>HHHHHHENLYFQGDTKEQRILNHVLQHAEPGNAQSVLEAIDTYCEQKEWAMNVGDKKGKIVDAVIQEHQPSVLLELGAYCGYSAVRMARLLSPGARLITIEINPDCAA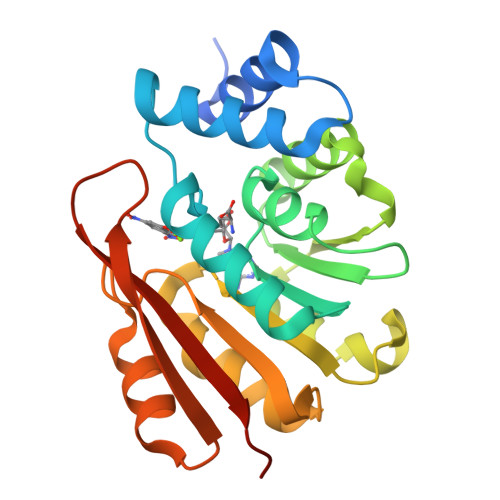ITQRMVDFAGVKDKVTLVVGASQDIIPQLKKKYDVDTLDMVFLDHWKDRYLPDTLLLEECGLLRKGTVLLADNVICPGAPDFLAHVRGSSCFECTHYQSFLEYREVVDGLEKAIYKGPGSEAGP[2x]> MKTQIGYFASLEQYRPMDALEQAIRAEKVGFDSVWVDDHFHPWYHDNAQSAQAWAWMGAALQATKKVFI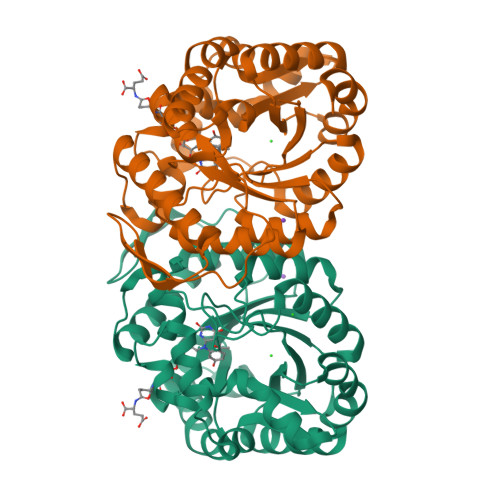STCITCPIMRYNPAIVAQTFATLRQMYPGRVGVAVGAGEAMNEVPVTGEWPSVPVRQDMTVEAVKVMRMLWESDKPVTFKGDYFTLDKAFLYTKPDDEVPLYFSGMGPKGAKLAGMYGDHLMTVAAAPSTLKNVTIPKFEEGAREAGKDPSKMEHAMLIWYSVDPDYDKAVEALRFWAGCLVPSMFKYKVYDPKEVQLHANLVHCDTIKENYMCATDAEEMIKEIERFKEAGINHFCLGNSSPDVNFGIDIFKEVIPAVRD methyl-9Z,12Z,15Z-octadecatrienylphosphonofluoridate | C19 H34 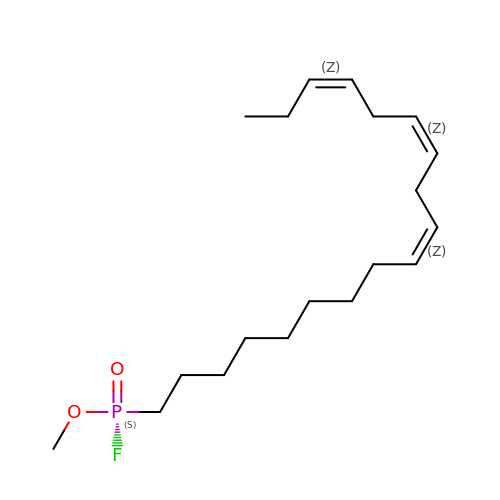F O2 P | MEHJVKGETWKOKY-SINQZMEQSA-N> MAGSGSERAEHQIILPESHLSSPLVKHKLLYYWKLTGLPLPDECDFDHLILSRQWKKILESSTPDIERMIKLGRSVHQTLSHSSKLTGILHPRCLEDLVGLDIPDSTNKFRRIEKKIQIHNTRYGEPF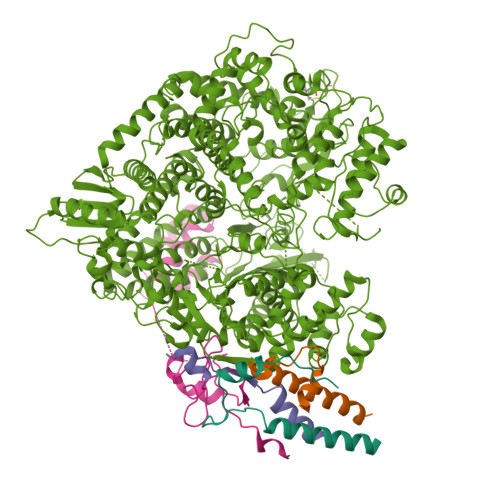TRLCSYVEKKLLGSSWTHKIRRSEEFDSLRTDPAFWFHSSWSTAKFAWLHVKQIQRHLIVAARTRSASNKLVTLSHRSGQVFITPELVIVTHTNENKFTCLSQELVLMYADMMEGRDMVNIISSTAVHLRCLAEKIDDILRLVDALARDLGNQVYDVVALMEGFAYGAVQLLEPSGTFAGDFFSFNLQELRDTLICLLPQRIADSVTHAIANIFSGLEQNQAAEMLCLLRLWGHPLLESRAAAKAVRAQMCAPKMVDFDMILQVLSFFKGTIINGYRKKNAGVWPRVKAHTIYGNVIAQLHADSAEISHDIMLREYKNLSAIEFEACIEYDPVTNLSMFLKDKAIAHPRNNWLASFRRNLLSEEQKKNVQDSTSTNRLLIEFLESNDFDPYKEMEYLTTLEYLRDDSVAVSYSLKEEEVKVNGRIFAKLTKKLRNCQVMAEGILADQIAPFFQGNGVIQDSISLTKSMLAMSQLSYNSNRKRITDCKERVSSSRNHDLKGKHRRRVATFITTDLQKYCLNWRYQTIKLFAHAINQLMGLPHFFEWIHLRLMDTTMFVGDPFNPPSDPTDYDLTKVPNDDIYIVSARGGIEGLCQKLWTMISIAAIQLAAARSHCRVACMVQGDNQVIAVTREVRPDDSPESVLTQLHEASDNFFRELIHVNHLIGHNLKDRETIRSDTFFIYSKRIFKDGAILSQVLKNSSKLVLVSGDLSENTVMSCANISSTVARLCENGLPKDFCYYLNYLMSCIQTYFDSEFSITSSTQSGSNQSWINDIPFIHSYVLTPAQLGGLSNLQYSRLYTRNIGDPGTTAFAEVKRLEAVGLLGPNIMTNILTRPPGNGDWASLCNDPYSFNFESVASPSIVLKKHTQRVLFETCSNPLLSGVHTEDNEAEEKALAEYLLNQEVIHPRVAHAIMEASSVGRRKQIQGLVDTTNTVIKIALSRKPLGIKRLARIINYSSMHAMLFRDDVFLSNRANHPLVSSDMCSLALADYARNRSWSPLTGGRKILGVSNPDTIELVEGEILSISGGCSKCDSGDEQFTWFHLPSNIELTDDTSKNPPMRVPYLGSKTQERRAASLAKIAHMSPHVKAALRASSVLIWAYGDNDINWTAALKLARSRCNISSEYLRLLSPLPTAGNLQHRLDDGITQMTFTPASLYRVSPYVHISNDSQRLFTEEGVKEGNVVYQQIMLLGLSLIESLFPMTVTKTYDEITLHLHSKFSCCIREAPVAVPFELTGVAPDLRVVASNKFMYDPNPVAEGDFARLDLAIFKSYELNLESYSTVELMNILSISSGKLIGQSVVSYDEETSIKNDAIIVYDNTRNWISEAQNSDVVRLFEYAALEVLLDCSYQLYYLRVRGLNNVVLYMSDLYKNMPGILLSNIAATISHPIIHSRLHTVGLISHDGSHQLADTDFIELSAKLLVSCTRRVVSGLYAGNKYDLLFPSVLDDNLNEKMLQLISRLCCLYTVLFATTREIPKIRGLPAEEKCAMLTEYLLSDAVRPLLSPEQVDSITSPSIVTFPANLYYMSRKSLNLIREREDRDSILALMFPQEPLFEFPLVQDIGARVKDQLTMKPAAFLHELDLSAPARYDAYTLEQARSDCALADMGEDQLVRYLFRGVGTASSSWYKASHLLSVPEIRCARHGNSLYLAEGSGAIMSLLELHIPHETIYYNTLFSNEMNPPQRHFGPTPTQFLNSVVYRNLQAEVPCKDGFVQEFRTLWRENTEESDLTSDKAVGYITSVVPYRSVSLLHCDIEIPPGSNQSLLDQLATNLSLIAMHSVREGGVVIVKILYSMGYYFHLLVNLFTPCSVKGYVLSNGYACRGDMECYVVFVMGYLGGPTFVNEVVRMAKTLIQRHGTLLAKSDETALMALFTSQKQRVDNILSSPLPRLAKLLRRNIDTALIEAGGQPVRPFCAESLVNTLSDITQTTQVIASHIDTVIRSVIYMEAEGDLADTVFLFTPYNLSIDGKKRTSLKQCTRQILEVTILGLGPEDLNRVGDIISLILRGTISLEDLIPLRTYLKMSTCPKYLKSVLGLTKLREMFSDGSMLYLTRAQQKFYMKTVGNAVKGYYNSSKNENLYFQG;>[4x]MATFTDAEIDELFETSGTVIDSIITAQGKPVETVGRSAIPQGKTKALSLAWEKHGNTNTPAAQESAGEQDQHGQNQASNSNRATPEEGPHSSQAQAATQPQEDANESQLKTGASSSLLSMLDKLSNKSSNAKKGPPQSPPQQALHSKGSPAVEQTQHGANQGRAQQETGHQAAPSPGPPGTGVNIAFPGQRGVSPQSVGATQPAPQSGQNQGSTPASADHVQPPVDFVQAMMSMMEAISQRVSKIDYQLDLVLKQTSSIPTMRSEIQQLKTSVAVMEANLGMMKILDPGCANVSSLSDLRAVAKSHPVLIAGPGDPSPYVTQGGEIALNKLSQPVPHPSDLIKHATSGGPDIGIERDTVRALILSRPMHPSSSSKLLSKLDSAGSVEEIRKIKRLALNG>[2x]GSMGKDEALEKDLNDVSKEINLMLSTYAKLLSERAAVDASYIDEIDELFKEANAIENFLIQKREFLRQR

Meiosis protein TEX12 is an essential component of the synaptonemal complex (SC), which mediates homologous chromosome synapsis. It is also recruited to centrosomes in meiosis, and aberrantly in certain cancers, leading to centrosome dysfunction. Within the SC, TEX12 forms an intertwined complex with SYCE2 that undergoes fibrous assembly, driven by TEX12’s C-terminal tip. TEX12 undergoes conformational change upon C-terminal tip mutations, indicating that the sequence responsible for driving SYCE2-TEX12 assembly within the SC also controls the oligomeric state and conformation of isolated TEX12.

The increased solubility of TEX12 ΔCtip and FFV mutants at high concentrations enabled their crystallisation and structure solution by X-ray crystallography. The tetramer consists of two symmetry-related copies of two unique TEX12 chains that have subtle differences in side-chain positions (r.m.s. deviation = 0.58 Å). The interfaces between symmetry-related and unique chains are distinct, and on the basis of subsequent data, were designated as dimer and tetramer interfaces, respectively. The centre of the TEX12 ΔCtip tetramer, which have named the ‘hinge’ (for subsequent reasons), is characterised by reciprocal salt bridges between R78 and D82 amino-acids, in which extended arginine residues act as struts that provide increased local separation (of approximately 12 Å) between chains of the dimer interface. The hydrophobic core surrounding the hinge includes Y71 residues and is continuous with lateral four-helical bundles at both ends of the molecule. The four-helical bundles are stabilised by heptad interactions between chains in the dimer and tetramer interfaces, which also contribute to hydrophobic cores. Further, the ΔCtip SAXS scattering curve was closely fitted by the ΔCtip tetrameric crystal structure upon addition of the few missing C-terminal amino-acids (χ2 = 1.54), confirming that the ΔCtip crystal structure is representative of its tetrameric structure in solution. Thus, we conclude that TEX12 ΔCtip forms the anti-parallel tetramer observed in its crystal structure, albeit prone to concentration-dependent dissociation, and the same tetrameric structure is stabilised within TEX12 FFV by Ctip coiled-coils ‘tying-off’ both ends of the molecule. TEX12 ΔCtip and LFIL dimers form tetramers through the same interfaces, but lack stabilising Ctip coiled-coils, owing to their deletion (ΔCtip) and disruption (LFIL).> GSMKTNLKGETALHRACINNQVEKLILLLSLPGIDINVKDNAGWTPLHEACNYGNTVCVQEILQRCPEVDLLTQVDGVTPLHDAL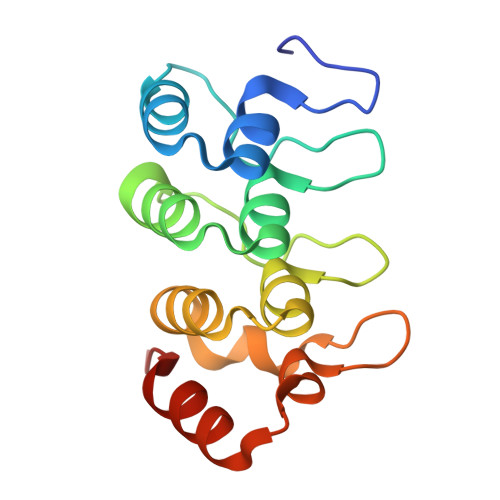SNGHVEIGKLLLQHGGPVLLQQRNAKGELPLDYVVSPQIKEELFAITKIED> MRSQIQSFLKTFEVRYPIIQAPMAGASTLELAATVTRLGGIG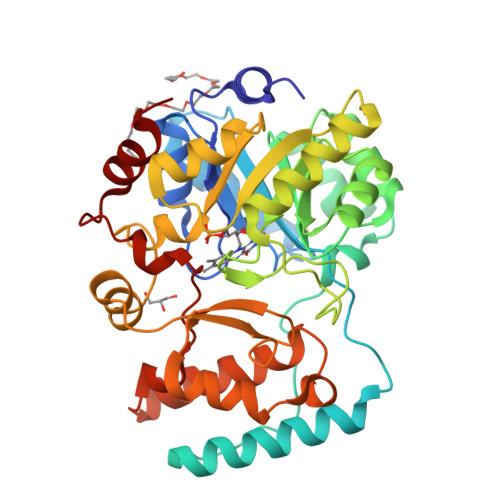SIPMGSLSEKCDAIETQLENFDELVGDSGRIVNLNFFAHKEPRSGRADVNEEWLKKYDKIYGKAGIEFDKKELKLLYPSFRSIVDPQHPTVRLLKNLKPKIVSFHFGLPHEAVIESLQASDIKIFVTVTNLQEFQQAYESKLDGVVLQGWEAGGHRGNFKANDVEDGQLKTLDLVSTIVDYIDSASISNPPFIIAAGGIHDDESIKELLQFNIAAVQLGTVWLPSSQATISPEHLKMFQSPKSDTMMTAAISGRNLRTISTPFLRDLHQSSPLASIPDYPLPYDSFKSLANDAKQSGKGPQYSAFLAGSNYHKSWKDTRSTEEIFSILVQDL> GSHMLEDPGAVTGPRKGGSRRNAWGNQSYAELISQAIESAPEKRLTLAQIYEWMVRTVPYFKDK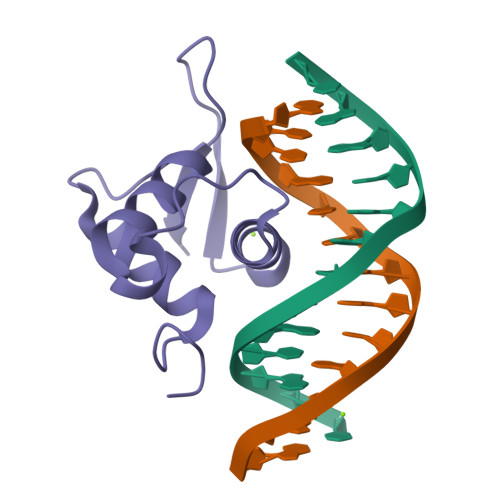GDSNSSAGWKNSIRHNLSLHSKFIKVHNEATGKSSWWMLNPEGGKS>IVGGYTCEENSLPYQVSLNSGSHFCGGSLISEQWVVSAAHCYKTRIQVRLGEHNIKVLEGNEQFINAAKIIRHPKYNRDTLDNDIMLIKLSSPAVINARVSTISLPTAP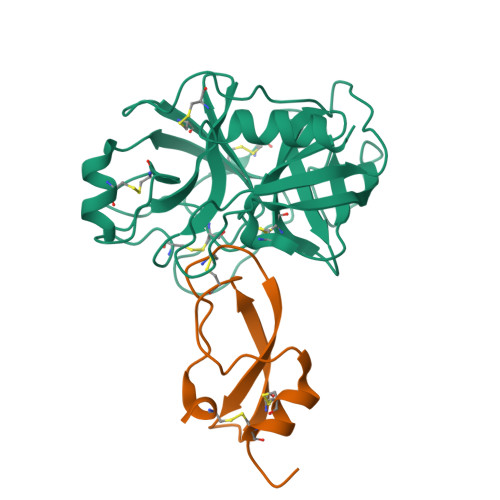PAAGTECLISGWGNTLSFGADYPDELKCLDAPVLTQAECKASYPGKITNSMFCVGFLEGGKDSCQRDAGGPVVCNGQLQGVVSWGHGCAWKNRPGVYTKVYNYVDWIKDTIAANS[4x];>[4x]EVCSEQAETGPCKAMISRWYFDVTEGKCAPFFYGGCGGNRNNFDTEEYCMAVCGSAI>[2x]CGADSQGLVVSFYTPATDGATFTAIAQRCNQQFGGRFTIAQVSLPRSPNEQRLQLARRLTGNDRTLDVMALDVVW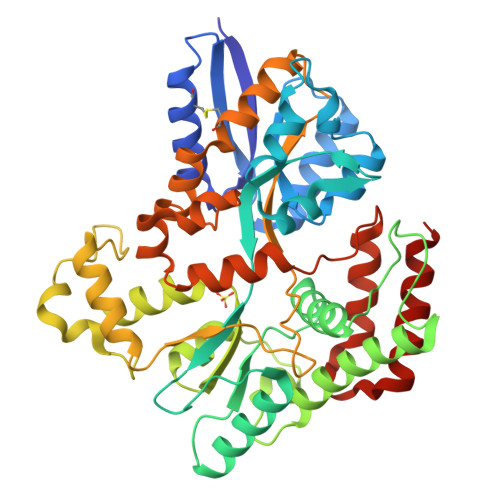TAEFAEAGWALPLSDDPAGLAENDAVADTLPGPLATAGWNHKLYAAPVTTNTQLLWYRPDLVNSPPTDWNAMIAEAARLHAAGEPSWIAVQANQGEGLVVWFNTLLVSAGGSVLSEDGRHVTLTDTPAHRAATVSALQILKSVATTPGADPSITRTEEGSARLAFEQGKAALEVNWPFVFASMLENAVKGGVPFLPLNRIPQLAGSINDIGTFTPSDEQFRIAYDASQQVFGFAPYPAVAPGQPAKVTIGGLNLAVAKTTRHRAEAFEAVRCLRDQHNQRYVSLEGGLPAVRASLYSDPQFQAKYPMHAIIRQQLTDAAVRPATPVYQALSIRLAAVLSPITEIDPESTADELAAQAQKAIDGMGLLP>MASWSHPQFEKGAETAVPNSSSVPGDPSSMPNPTSIEWRPSGKRPNVLLISADQWRGDCLSAVGHASVKTPNVDALAQDGVLFTRHFA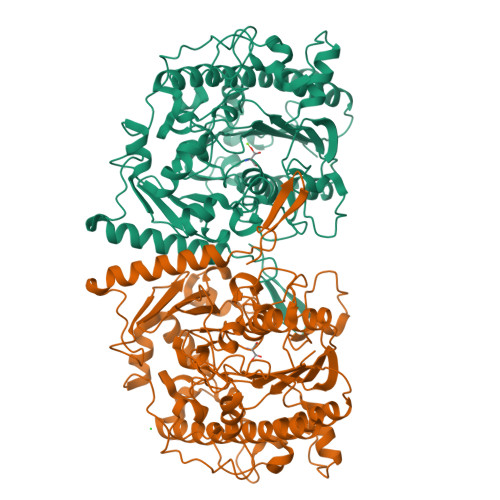GTAPASPARATLYTGLYQMNHRVCRNGSPLDARFDNLALAARRGGYDPTLFGYTDTAPDPRGMDPNDPHLTTYEGVLPGFSARQLLPEHEKQWLSWLRSRGHPEATSRDIHIPVGATPGEISDVAPAYSKDETQTAFLAGEFIRWLGEQDAPWFAHVSFLRPHPPFSVPEPYNRMFTPSDGPAFARAANREAEQAVHPLLAFALPLIGKDSFIYGGEGSASDWTSEDLSAIRAIYYGMIAEVDTQLGRIWQALKNVGAWDDTLIIFTSDHAEMMGDHWMLGKGGFFDGSYHVPLVIRDPGHPGGAGRQVERFTSAADIFPTLCDRLGLVPDNHLDGGTLVPFLEGGEPEGWRDAAFWEFDFRDIAKGEAERHFGLKSNACNLAVIRDERFKYVHFAGLPPLLYDLAKDPMELTNVAADADYAAVRLGYAEKLLSLRAQHLDQTLAYTELTEKGPVSRRP[4x]>MFLAKSIVCLALLAVANAQFDTNYASGRSGMVHLFEWKWDDIAAECENFLGPNGYAGVQVSPVNENAVKDSRPWWERYQPISYKLETRSGNEEQFASMVKRCNAVGVRTYVDVVFNHMAADGGTYGTGGSTASPSSKSYPGVPYSSLDFNPTCAISNYNDANEVRNCELVGLRDLNQGNSYVQDKVVEFLDHLIDLGVAGFRVDAAKHMWPADLAVIYGRLKNLNTDHGFASGSKAYIVQEVIDMGGEAISKSEYTGLGAITEFRHSDSIGKVFRGKDQLQYLTNWGTAWGFAASDRSLVFVDNHDNQRGHGAGGADVLTYKVPKQYKMASAFMLAHPFGTPRVMSSFSFTDTDQGPPTTDGHNIASPIFNSDNSCSGGWVCEHRWRQIYNMVAFRNTVGSDEIQNWWDNGSNQISFSRGSRGFVAFNNDNYDLNSSLQTGLPAGTYCDVISGSKSGSSCTGKTVTVGSDGRASINIGSSEDDGVLAIHVNAKL[2x]

Drosophila melanogaster α-amylase, DMA, which belongs to the glycoside hydrolase family 13, sub family 15, has been studied from an evolutionary, biochemical, and structural point of view. Indeed, plant produced inhibitors are an important element of the plant defense response to insect predation against feeding. α-Amylases (α-1,4-glucan-4-glucanohydrolase, EC 3.2.1.1) belong to the glycoside hydrolase family 13 (GH13) as classified in the CAZy database, and catalyze the hydrolysis of starch and related α-1,4-linked glycosyl polysaccharides. As reported for other α-amylases from mammals, insect, plants, fungi, archaea and bacterial α-amylases, the enzyme consists of three distinct domains, A (residues 1 to 97 and 160 to 379), B (residues 98 to 159) and C (residues 380 to 476). In DMA, the nucleophile is Asp186, the general acid/base catalyst Glu223 and the transition state stabilizer is Asp288.

The three-dimensional structure of DMA in complex with the well-known α-glucosidase inhibitor acarbose was solved to 2.0 Å resolution. Several studies have reported transglycosylation reactions taking place within α-amylase crystals, in particular when using the pseudo-tetrasaccharide acarbose as ligand. For the DMA-acarbose complex, careful inspection of the electron density maps in the active site region revealed a well-defined heptasaccharide occupying subsites −4 to +3 resulting from a transglycosylation reaction as seen for the psychrophilic AHA and the human salivary α-amylase, HSA. As observed for other α-amylases, this insect α-amylase performs transglycosylation reactions when in the presence of the anti-diabetes pseudo-tetrasaccharide drug, acarbose, under water poor conditions. Hereby, the pseudo-tetrasaccharide which is synthesized by Actinoplanes sp. and which is composed of an acarviosin linked to maltose, is transformed to a heptasaccharide consisting of an acarviosin-glucose linked to an acarbose. In addition to this structural calcium ion, a second metal ion, which is located between the catalytic domain A and domain C, was revealed in the DMA crystal structures described herein. It is interesting to notice that the only direct coordination of this putative calcium ion to the protein is via Gln263, an amino acid residue which is only conserved in the subgroup of D. melanogaster and which is not present in other animal α-amylases.>[4x]MKVLVTGFEPFGGEKINPTERIAKDLDGIKIGDAQVFGRVLPVVFGKAKEVLEKTLEEIKPDIAIHVGLAPGRSAISIERIAVNAIDARIPD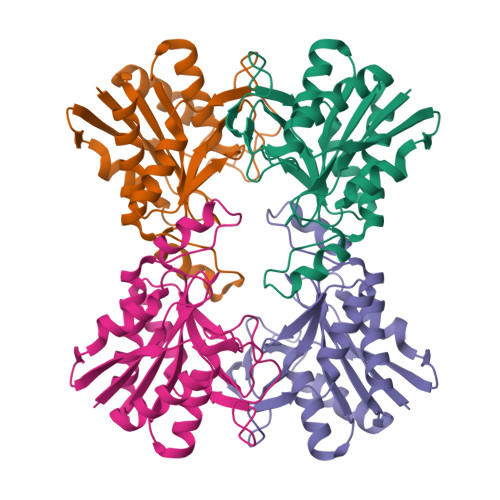NEGKKIEDEPIVPGAPTAYFSTLPIKKIMKKLHERGIPAYISNSAGLYLSNYVMYLSLHHSATKGYPKMSGFIHVPYIPEQIIDKIGKGQVPPSMSYEMELEAVKVPIEVALEELL> GPMRAIDL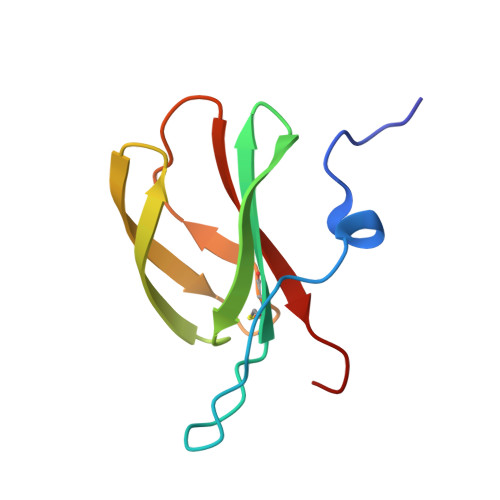SRERDPNFFDNADIPVPECFWFMFKNNVRQDAGTCYSSWKMDKKVGPNWVHIKSDDNCNLSGDFPPGWIVLGKKRPGF> GHMRYEDAYQYQNIFGPLVKLEADYDKKLKESQTQDNITVRWDLGLNKKRIAYFTLPKTDSDMRLMQGDEICLRYKGDLAPLWKGIGHVIKVPDNYGDEIAIELRSSVGAPVEVTHNFQVDFVWKSTSFDRMQSALKTFAVDETSVSGYIYHKLLGHEVEDVIIKCQLPKRFTAQGLPDLNHSQVYAVKTVLQRPLSLIQGPPGTGKTVTSATIVYHLARQGNGPVLVCAPSNIAVDQLTEKIHQTGLKVVRLCAKSREAIDSPVSFLALHNQIRNMDSMPELQKLQQLKDETGELSSADEKRYRALKRTAERELLMNADVICCTCVGAGDPRLAKMQFRSILIDESTQATEPECMVPVVLGAKQLILVGDHCQLGPVVMCKKAAKAGLSQSLFERLVVLGIRPIRLQVQYRMHPALSAFPSNIFYEGSLQNGVTAADRVKKGFDFQWPQPDKPMFFYVTQGQEEIASSGTSYLNR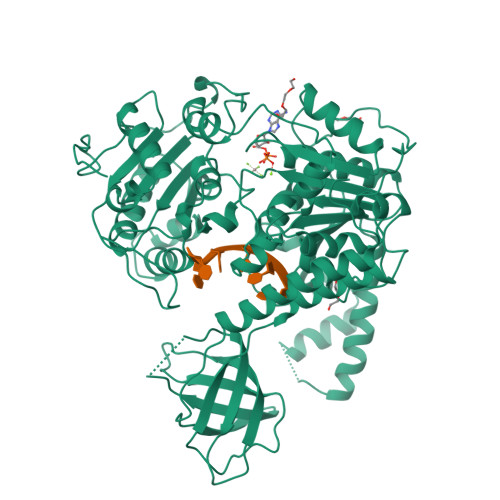TEAANVEKITTKLLKAGAKPDQIGIITPYEGQRSYLVQYMQFSGSLHTKLYQEVEIASVDAFQGREKDFIILSCVRANEHQGIGFLNDPRRLNVALTRARYGVIIVGNPKALSKQPLWNHLLNYYKEQKVLVEGPLNNLRESLMQFS>[2x]MTQDELKKAVGWAALQYVQPGTIVGVGTGSTAAHFIDALGTMKGQIEGAVS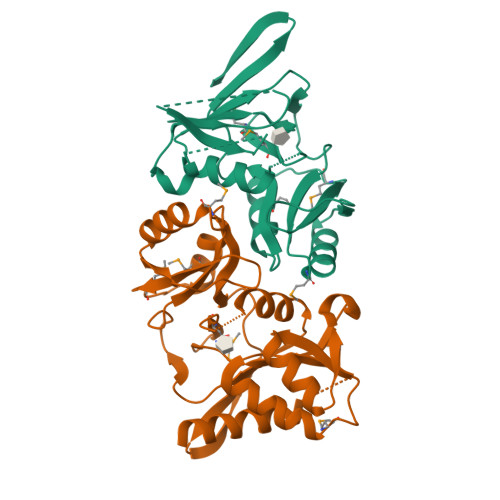SSDASTEKLKSLGIHVFDLNEVDSLGIYVDGADEINGHMQMIKGGGAALTREKIIASVAEKFICIADASKQVDILGKFPLPVEVIPMARSAVARQLVKLGGRPEYRQGVVTDNGNVILDVHGMEILDPIAMENAINAIPGVVTVGLFANRGADVALIGTPDGVKTIVK>MLEDLKRQVLEANLALPKHNLVTLTWGNVSAVDRERGVFVIKPSGVDYSIMTADDMVVVSIETGEVVEGAKKPSSDTPTHRLLYQAFPSIGGIVHTHSRHATIWAQAGQSIPATGTTHADYFYGTIPCTRKMTDAEINGEYEWETGNVIVETFEKQGIDAAQMPGVLVHSHGPFAWGKNAEDAVHNAI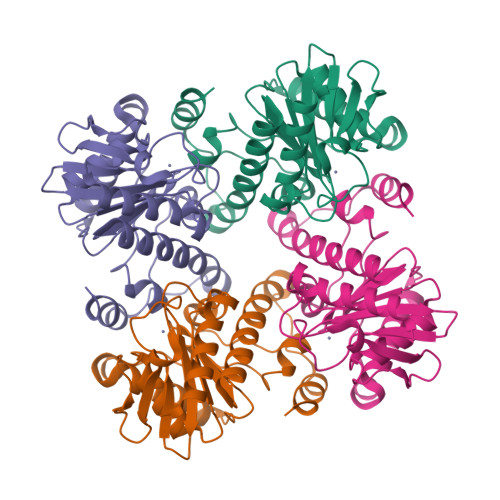VLEEVAYMGIFCRQLAPQLPDMQQTLLNKHYLRKHGAKAYYGQ[6x]>[2x]TDTTPPTITLPQEVIAYRGEEFEFFVETTDDSGRVNRVIVRNIEGADNSTYLDPNWIRYSTDNLSVPGNATPANPLRTRVYGIVPINHGVGPGDRYTKYVRAEDAAGNITALVDKQSERFVLVIRPQTEKYTPQVPTLTYVQNANSLTQTDKDAVI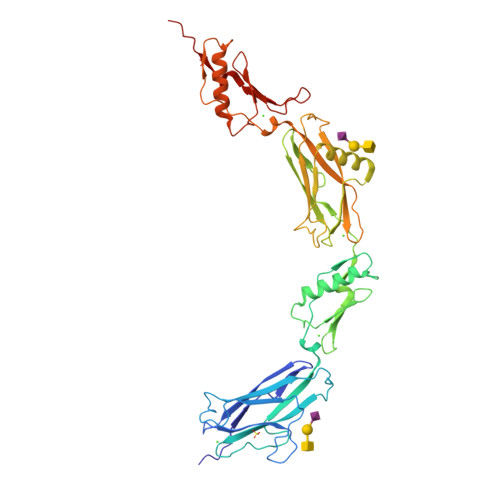AAVKSANPNLPATSTYSVSENGTVTITYPDGSTDTIAAAQTVDTDRVAPVFVDEGRDYIFYRGEEGTAELHFYDNSGKITNVNFAGDLAASSTYNTLLGLGFTFNTPNINNPNNATEQNPLVTTIRGTIPKSLPAGPGGKYTFKVRATDASGLTSEAKIFRIVFANQTDKYTPNNPGSLTGVLNPQQLSTSEKTAIEEKVRAANTGNLPNNVQYVVNNDGSVTVIYPDDTPASRSRDTITADRTVQDLRPRNS> MLSSKYSKRIAWMKTTICDSLQLKDMIVEESFQYEKNKNLLEQFLSGEGLNKIFAYYQVQEQAQNDDIKDTGAQDPVLFFTTGDLEKIQDKAVWFLRITNPADDKKKASQQDGNDNDIIFGEITPNTVPMLNALMESVYSRQIDHIITEKIQFWGVAEEEQVLEFQQHS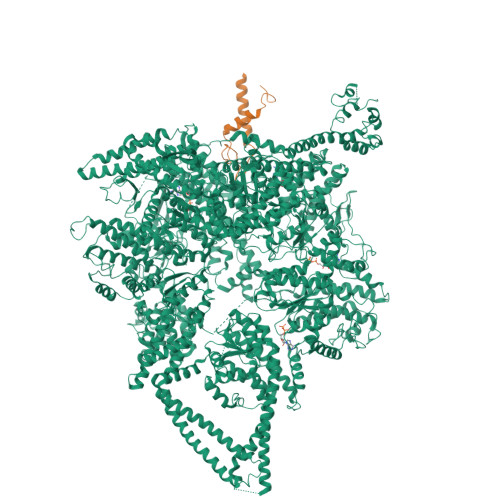NKFSSEVREAINLMSPGTEHFKLDYEAISGLSESEKMQHYEMKFNEWINLISSQLNDDSEVRKDEKDAGPATELIYWRSRMQKITNWSEQLKSKDFQIVKASLQRHKNHDNQRPRGDESLSKLMMEYNRLDLLLTDKLNEAKDNVKYLTTLEKFIEPLYNGTPQQIIDTLPALMNAIKMIHTIARFYNTTDKMTGLFIKITNQMIKNCKDRILNKKDNGDNPSLYKMIWEQDPAELIEVLGSCIKLYCEYKKCYNDTKEKVADMPKGKTFDFSDAQIFGKFDTFVRRLQKLIEIFSNIQQFNALAKHNLEGMDVLTNKFKKIIDDFKKKGHNLLDTANNKFDRDWVEFNVEISHLDGELQNFIDNNFNRFRNIEYSLKLLHKFQSTIKRDSLKHNLTSRYNAILHNYATELDTIQRVFQDQKSNPPLVRNMPPEAGKIIWARHLFQKITGPINIFPENVINSTEIRRYYGSYNTLGKQLTIYEMWFYQDWVNKIEQSKAALQATLIVRHDENKKLYVNFDLEIMQLIREAKCLDRQGIEIPESARIILLQEDKFKTYYNELLYALKEYERINSKIKPICKNLLLPHIEDLDLKLRPGMVTLTWTSMNIESYLYYVHQGLKKLEQLIINVNDIIENRIENNLKTVSKVVLVHLPQDTKPLSLDSFVQLQEEYINSKTDFLTSKNVEVERAVDDLLQTIMLYPLDPHVDPVLPEETKRIKRYYFWYFYQALLNSTQNSLNAMKYRVCGKKIPGANTLQNLKPFFQVEVQLNGDKVTLNPSLQEIQKSINRAATAVLRCSKHLYNWDQQNKDSTDKATFYDMIACDKEIVKVILLLTGSIQGTKNKVNEFLSGFTKFEWLCKESIQESIKKFSKNGPTLQNYEDQLKKFSQIEEEIEKIVPTYKIGAMELMTHNICTSLSTWAKEWKLQYSQDLHKRARQLLDSLTEQTKMLSTKLSKPVKDIDSLGYVMETLEQIRKEQAEIDMKFNPVQEMYSLLDNYLPGGITDKDEMDARSLLRRNWDILIQQAEIKGKEYQHKQAIYLKELKQSIKDFTNQVSIFRRDYEKNGPMVEGISPAEAMERLRRFEDEYDVKYQMYKINARGENLFGLQNQKYPELEKTDAEIKNLNKLYNLYDSVIKNIQQFKEKSWQDVSKDDLAKMEEDAGKYGEQCSRLPKDLKEWQAYRDLKNYIDSLREQLPLIISLKKPSIMPRHWEKIKEITNTKLNYENPDQFYIEEIMGAKLLDFREDIEDITESADKQLKIRTGLDEINLYWNDMQFQFGIWGKRDVPCMLNGLIVGTILERLEEDQLQLSTFNSQRHVTPFKAEVENLIRTFSDVNDTLDMWVKVQKLWTSLEPVFTGGDIARQMPLQAKQFQGIDKNWMKIMEKAVETKKVIPCCQNDMLKDFLPDLNRKLEDCQKMLEAYLEGKRKKFPRFYFVSNPTLLKILSQGSEPTSIQEDFEKLFDAITKVTFESAKDKKNPALKQITQIQQVIGRNEENISLTGYYVKCEGNIEDWLKKLEQNMQQTLKDIASAAAQQVFQVGLKEFVSSQASQIALLGLQILWTSKVNEGLERLSRNERNAMDIKRNEIKEHMNILSSMCLEDLNGAVERTKVETLVTIQVHQKDISMDLKCKDVNDFEWQKQTRIAWKTDIDECIISITDWDSPYSYEFLGAKERLCITPLTDRCYITLAQAMSMYYGGAPAGPAGTGKTETVKDLGRTLGVFVVVTNCSDQHRYRDMAKIFKGLVQSGLWGCFDEFNRIDLEVLSVVAMQVESITTARKQHMKKFMFPEEEIEIELIPTVSYFITMNPGYAGRQELPENLKVLFRGVSMMVPDREIIIKVKLASVGYLQIDLLAKKFNVLYRLCEEQLSKQRHYDFGLRNILSVLRTAGNTKRQEIKSDEEMLLMRSLRDMNLSKLVADDIPLFNGLLADIFPKLKEVPKKLYPDVEKKIPEEINAESYLINTPSFQLKIIQLYETCLVRHGFMLVGPTGSGKSTIMKILTEVLTKLGSPHKIVIMNPKAITAEQMYGVKSEISDDWIPGVFSTIWAKSNNRALKHTTWITCDGPVDAIWIENLNTVLDDNKILTLANGERIAMTENCKVVFEVENLNNASPATVSRCGQVYVSPTDLGYEAVIEGWIRNRKASGRAEESDKLGNILRKYLINMRFIELQSKECKEPMMDTSPVISVINILNLLTGCLQYFVQTQRTLSEQEYEKFIVYSMAWAIGGIYEAQDRVRFHELLLAKNAPIPQKGKENETVFDYYVSQDYLDWKICSPEEWVPPQSLQFSQLLLPTLDSFRAEMLLNFILTQPKSHTCSNSALLIGGSGTAKTSSVLLYCNKFDPQKMLFKRTNFSSATSPFMFQSTIEAECDFKVGKEFAPPGNKMMTIFIDDMSMPFVNKWGDQITLELVRQLIETGGFYMLDKTQRGNQRKMKNLQYIGAMNHPGGGRNDIPNRLKRQFFIFNMILPLSIEGIYGPIIKHMFKQKYFSDSTYKVIESLTSATIALWNKVKSTMLPTPAKFHYVFNMRELSRIFKGILTCKKDTINDAPKSMKIKPELFLVGLWRHEAERVLADKLVNNKDKDTVMGYIQEVSLESFSQIENEILEKYSSEKTFLFCDFLRPDVINEDGIIEEEAPKIYEAIDSLTELRKRCNFLLSFYNDRNPSKKMPLVLFDDALKHLLRISRIIRQPRSSGLLVGVGGSGKQSLTRLAGFIGKNLIQQIIVTKTYSDKDLKEDIKKGFDDAGHLGKQVTFLMTDSEVKKEEFLEYINMVLSTGEIPNLLAKDEREVWLGDISQAYCKEKNLGNIDPPQSELWTYFVDRVRDNFHIMLCFSPVGQKFRERARKFPALFNECTIDWFLPWPEEALVSVAETFIKNFDKLDTKEETKQELMKHMGNVHLMVNEICDEYYQKMRRQVYVTPKSFLSYLNSYKTLYIEKYDELDQQEESFKIGLNKIQEATITINQMEISLKEEEIQLNEATEKTNQLLANLDKESKKANQKGEEVAATNKQCEIQAEQISKEKEEAERELEAALPALRRAQEAVDSIESKDIVELKANKKPLDIIKYIMDAVLVFFKARLIPIQIEERVFNKKEGKAVLFLKESYDESGIQTLGDMNFMKKLKEFEKDSINEETIELLEPYLNQSEDWFNDTFATKASKAAAGILKWAFAIYEYHQKSKIVKPKRIQVAIAEGRQAIALKELEKAREDLAQIQAYIKNLKDVYTKQMEEKNELEMKAAKTKKKINTARTLITSLSGEKDRWGKGAQDISDQKRKLVGNVSLSTAFISYCGPFNAEYRNKLAQQRFVVDMKKRGVPVTPGLELTSFLIDDATIGEWNLQGLPKDDLSIQNGIMVTNSARYPLFIDPQGQGQNWIRNKLSASIIPERCITTLSHPKFKDMFLKYCMESGLTLIVENIENEVDPMMDPVLERQIIVKGKTQFVNVAGTEMELSKEFKLFMTCRLANPSFSPELSAKTTIIDFTVTQSGLEQQLLGKVISKEQKALEDSLNQLLADVNQNQKDLQRLDKNLLERLINSQGNLLDDTELMDVLNNTKTQAKEVAAKLIDAEIKTKEINEKREQYRPVAIRGSAIYFTMIEVSLVNWMYNSSLEQFLKLFIESIDLSEKAQLPSNRVKNIISFLTFHVYRYVNRGLFEKDKITFILMMAFKILTTAGTISSGDVSLFLKSGDALDIKSERQKQISYLEDNQWLNILALSKHTFSGQTLPFFKELPDLISRSENQWRNWIDKNDPENFPIPDFAESINQEKEIGSFISLCLVRSLRNDRTLIATQNFISNVLGKEFTDPISYPIEGIWQESSNMDPVLFLLSAGADPTSSIDELAKKKKKFPCEKVSMGEGQERVARQVIMKGFVEGGWVILQNCHLGLKFMEEIETLVSPINQIHEDFRLWITCEQHPKFPLGLLQKTLKVTNEPPKGLKAGLYKTFTTIITQEFIDKVDHSNWRSLIFTICFLHSIVIERKKFGPLGWCVPYEYNYSDLEASLLYIEKYLTNLMSTPQPNSHNLPISMNVVRYMICEVQYGGRITDDLDRELFITYGETYLKDGIFGNDYFFYDIMVDGSGQKFKYRIPQNPSAELIKYQEYIAKVPTVDNPEVFGLHSNADLTFRLKESKEMINTVMETRPKDSSVGGGKTREEIVQDKAKDMLKNLPPDYNDVEVRELVSKLGGPNPKTSTERGMTVPLNIFLYQEVTRMQRVIGLVRKTLQDTILAIDGQIIMTPEILEAINAIYDAKVPNSWLYDPSGAEISWLLPNLGSWSTSLSDRNKQLNDWLRSGQRPILFWLTGFFNPQGFLTGMKQEVTRNHKKGDGKGGEAWSLDDVVYSTTVKEREKEKDIEQPPAEGVYIKGLYLEGCKWSKNGLDDSDPKKIFADLPILHVSAINKKKTNEQDRMSNTYLCPVYKYPKRTDKYLIFRVGLPCEGSNNPSHWKLRGVALLCSTE;> MFNFFSSANINQNIPKYSVNDFVFRLKKIEKIVVKEGLDGFLLINGVDSRENTEYVKLTNWLFLGNSGLEIEENEYLNQIYSDMIVLIKKGTTHIFIDPEALNSLQTLIYSIPNVDVFCPTEKQYEDKDEMELLKMAFFLRVMKPTKKVGILLGQKDKGKINSIEKWPLIQSYGLEELGVGFFSMNHEVVDLTLRLNAVYKNYDKFFVSKLIYVVAKRLTGHFNSAAGQLGDMKMHKRNLATESQLTEIFRDTYEIEEISKWVQIRGVNAALPKPRVLFGKNTSADCSKEPSVAPLKDLKYSETFHSFHATFETFDLRTCLRAARTYFLAKGVKEERNLITLNDDEGVPQGYELNIDENQQYKDQDFLANLYLSIIIGFNEVMQLITKDYKNMTEEFIQDYIFQKVSKVYAGFQIPESEITLDKIQIILKAYNSFGEEVKIDFKDTISFKLTPYFFMVRIEQKNIKSQILNNTVLGSLVFAESFILQEGCYLLLTKEIPYFDLWNCQNDYSEKIEKMKKRILWEPLGKQISDELPKNRIFVQTGRKSNYGFDIPIMQASYYMHELGLRIETQRLGWFILFFKEMKEIQITQKMNHTWLIFKVDSNITFNSISKDTIALEFTGDALEQSFFKIKNYFEENQIKYEYQVDIPAIFQESQIAKKQILNQQSQGQKLITMNSIQNEQFFISYIESKQLMILNQMKDLKLSAYKNLYEQMQISQAITPVENHIGVILVNGSYCSGKRKFAENLIRFGSDNNLRLHLYKFDLNEMSELTEKSYLSGLLKFASEKKIQNTDVIVASVPHFINTKILIDYFSKSEKISNAFYIRTIATKININNIYSNFNKNPVNNVFTYGVEGYSQFLLLDTYNNYDADVNALNKTLSGVLPGAKIYKIMNNILNPALAKDILTSITFISEQNNLNRLKYSVQYDLLTSNGPSSVVFIPFKLPILREKIRDLIYKKILQNGNQTLVDTIEAEQKIAEFKELNKNSKDPLMIEIIKLKEKIEIQNAQTSDQAIKIDYVKGILRYDSKLKEGLEEITITPNYFIERTVKGVDAKEFTEELNGVSFKNVKYTGITNSIINDMGFVFAGKNLNKEKLLELLYKLVKPLNKQKLRQRKDLTEEEIVDIQFRNRGEGLENGEFYDGQFWRNIQGLILPHHPKKDEFIEEYLKQEEVRINQINEQLQQEWETWKQVYDKIHLDK> MDGVSSEANEENDNIERPVRRRHSSILKPPRSPLQDLRGGNERVQESNALRNKKNSRRVSFADTIKVFQTESHMKIVRKSEMEGCSAMVPSQLQLLPPGFKRFSCLSLPETETGENLLLIQNKKLEDNYCEITGMNTLLSAPIHTQMQQKEFSIIEHTRERKHANDQTVIFSDENQMDLTSSHTVMITKGLLDNPISEKSTKIDTTSFLANLKLHTEDSRMKKEVNFSVDQNTSSENKIDFNDFIKRLKTGKCSAFPDVPDKENFEIPIYSKEPNSASSTHQMHVSLKEDENNSNITRLFREKDDGMNFTQCHTANIQTLIPTSSETNSRESKGNDITIYGNDFMDLTFNHTLQILPATGNFSEIENQTQNAMDVTTGYGTKASGNKTVFKSKQNTAFQDLSINSADKIHITRSHIMGAETHIVSQTCNQDARILAMTPESIYSNPSIQGCKTVFYSSCNDAMEMTKCLSNMREEKNLLKHDSNYAKMYCNPDAMSSLTEKTIYSGEENMDITKSHTVAIDNQIFKQDQSNVQIAAAPTPEKEMMLQNLMTTSEDGKMNVNCNSVPHVSKERIQQSLSNPLSISLTDRKTELLSGENMDLTESHTSNLGSQVPLAAYNLAPESTSESHSQSKSSSDECEEITKSRNEPFQRSDIIAKNSLTDTWNKDKDWVLKILPYLDKDSPQSADCNQEIATSHNIVYCGGVLDKQITNRNTVSWEQSLFSTTKPLFSSGQFSMKNHDTAISSHTVKSVLGQNSKLAEPLRKSLSNPTPDYCHDKMIICSEEEQNMDLTKSHTVVIGFGPSELQELGKTNLEHTTGQLTTMNRQIAVKVEKCGKSPIEKSGVLKSNCIMDVLEDESVQKPKFPKEKQNVKIWGRKSVGGPKIDKTIVFSEDDKNDMDITKSYTIEINHRPLLEKRDCHLVPLAGTSETILYTCRQDDMEITRSHTTALECKTVSPDEITTRPMDKTVVFVDNHVELEMTESHTVFIDYQEKERTDRPNFELSQRKSLGTPTVICTPTEESVFFPGNGESDRLVANDSQLTPLEEWSNNRGPVEVADNMELSKSATCKNIKDVQSPGFLNEPLSSKSQRRKSLKLKNDKTIVFSENHKNDMDITQSCMVEIDNESALEDKEDFHLAGASKTILYSCGQDDMEITRSHTTALECKTLLPNEIAIRPMDKTVLFTDNYSDLEVTDSHTVFIDCQATEKILEENPKFGIGKGKNLGVSFPKDNSCVQEIAEKQALAVGNKIVLHTEQKQQLFAATNRTTNEIIKFHSAAMDEKVIGKVVDQACTLEKAQVESCQLNNRDRRNVDFTSSHATAVCGSSDNYSCLPNVISCTDNLEGSAMLLCDKDEEKANYCPVQNDLAYANDFASEYYLESEGQPLSAPCPLLEKEEVIQTSTKGQLDCVITLHKDQDLIKDPRNLLANQTLVYSQDLGEMTKLNSKRVSFKLPKDQMKVYVDDIYVIPQPHFSTDQPPLPKKGQSSINKEEVILSKAGNKSLNIIENSSAPICENKPKILNSEEWFAAACKKELKENIQTTNYNTALDFHSNSDVTKQVIQTHVNAGEAPDPVITSNVPCFHSIKPNLNNLNGKTGEFLAFQTVHLPPLPEQLLELGNKAHNDMHIVQATEIHNINIISSNAKDSRDEENKKSHNGAETTSLPPKTVFKDKVRRCSLGIFLPRLPNKRNCSVTGIDDLEQIPADTTDINHLETQPVSSKDSGIGSVAGKLNLSPSQYINEENLPVYPDEINSSDSINIETEEKALIETYQKEISPYENKMGKTCNSQKRTWVQEEEDIHKEKKIRKNEIKFSDTTQDREIFDHHTEEDIDKSANSVLIKNLSRTPSSCSSSLDSIKADGTSLDFSTYRSSQMESQFLRDTICEES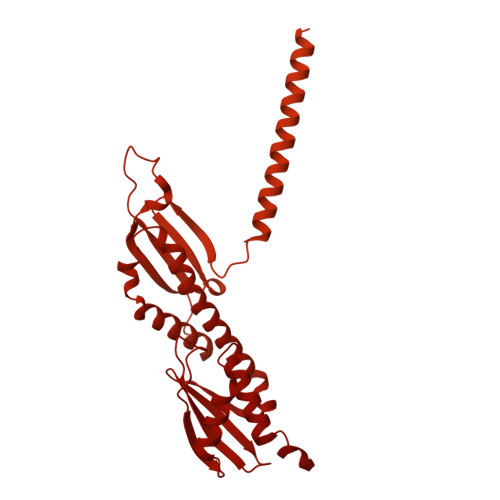LREKLQDGRITIREFFILLQVHILIQKPRQSNLPGNFTVNTPPTPEDLMLSQYVYRPKIQIYREDCEARRQKIEELKLSASNQDKLLVDINKNLWEKMRHCSDKELKAFGIYLNKIKSCFTKMTKVFTHQGKVALYGKLVQSAQNEREKLQIKIDEMDKILKKIDNCLTEMETETKNLEDEEKNNPVEEWDSEMRAAEKELEQLKTEEEELQRNLLELEVQKEQTLAQIDFMQKQRNRTEELLDQLSLSEWDVVEWSDDQAVFTFVYDTIQLTITFEESVVGFPFLDKRYRKIVDVNFQSLLDEDQAPPSSLLVHKLIFQYVEEKESWKKTCTTQHQLPKMLEEFSLVVHHCRLLGEEIEYLKRWGPNYNLMNIDINNNELRLLFSSSAAFAKFEITLFLSAYYPSVPLPSTIQNHVGNTSQDDIATILSKVPLENNYLKNVVKQIYQDLFQDCHFYH>MNNQCKTIAHVLRVNNGQELHVWETPPKENVPFKNNTILIASGFARRMDHFAGLAEYLSTNGFHVFRYDSLHHVGLSSGSIDEFTMTTGKNSLCTVYHWLQTKGTQNIGLIAASLSARVAYEVISDLELSFLITAVGVVNLRDTLEKALGFDYLSLPIDELPNDLDFEGHKLGSEVFVRDCFEHHWDTLDSTLDKVANTSVPLIAFTANNDDWVKQ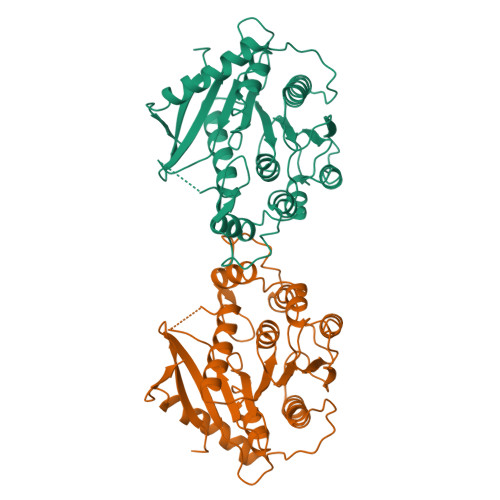EEVYDMLAHIRTGHCKLYSLLGSSHDLGENLVVLRNFYQSVTKAAIAMDGGSLEIDVDFIEPDFEQLTIATVNERRLKAEIENRTPEMA[2x]> SMPRDNMASLIQRIARQASLTFRGSGGGRGASDRDAASGPEAPMQPGFPENLSKLKSLLTQLRAEDLNIAPRKATLQPLPPNLPPVTYMHIYETDGFSLGVFLLKSGTSIPLHDHPGMHGMLKVLYGTVRISCMDKLDAGGGQRPRALPPEQQFEPPLQPREREAVRPGVLRSRAEYTEASGPCILTPHRDNLHQIDAVEGPAAFLDILAPPYDPDDGRDCHYYRVLEPVRPKEASSSASDLPREVWLLETPQADDFWCEGEPYPGPKVFP;> XYIVKTFWLGSHRQCX

N-terminal cysteine oxidases (NCOs) act as enzymatic oxygen (O2) sensors, coordinating cellular changes to hypoxia in animals and plants. They regulate the O2-dependent stability of proteins bearing an N-terminal cysteine residue through the N-degron pathway. In animals, the Cys branch of the N-degron pathway is regulated by the NCO 2-aminoethanethiol dioxygenase (ADO), which also plays a role in cysteamine catabolism and taurine biosynthesis. Biochemically, ADO is a non-haem iron-dependent thiol dioxygenase (TDO) from the cupin fold family of enzymes, consisting of a conserved double stranded β-helix (DSBH) core in which the active site is situated.

A crystal structure of ADO in complex with CP6 was obtained through co-crystallisation to characterise its binding mode and evaluate how differences in CP sequence can influence the means of inhibition. However, two crystal structures of unbound ADO, which were published during this investigation, highlighted alterations that result in an amenable crystallisation construct, including metal cofactor substitution and surface Cys mutations. CP6 adopts an antiparallel β-sheet conformation, which is maintained through a series of intramolecular hydrogen bonds between backbone and sidechain atoms. The peptide sits across one end of the DSBH core of ADO, blocking the active site entrance. CP6 binding is mediated by a number of intermolecular interactions, including pi-stacking between the sidechain of CP6-W7 and the sidechain of ADO-Y87, pi-stacking between the C-terminal amide of CP6-C14 and the sidechain of ADO-W257, and hydrogen bonds between the sidechain of CP6-R12 and the backbone carbonyls of ADO-Q252, -A253 and -F256. Additional changes in ADO structure are largely restricted to amino acid sidechains including, most notably, ADO-W257, which rotates to stack with the C-terminal amide of CP6-C14, and ADO-E92, which adopts a distinct conformation to avoid clashing with CP6-F6. Additional electron density is observed around the active site metal, which was modelled as Tris coordinating cobalt in multiple conformations. CP6-K4 and -F6 interact with ADO-D215 and ADO-E92, respectively. While there is no immediate rationale for the functional contribution of the former, CP6-F6 promotes formation of a hydrogen bonding network down to the active site via ADO-E92, -H89, -Y87 and a water molecule, which is not present in the peptide-free structure.> SKGENSKLNPWAVVGFIDAEGSFMVRVRKNSKYKTGWLVVAIFSVTVDKKDLFLLESLKTFFGGLGSIKKSGNSTFSYRIESSEQLTKIILPFFDKYSLITEKLGDYLLFKKVLELMGTKEHLTQRGLEKIVSLKASINKGLSEELQAAFPQCVPTPRPEINNKNIPDPFWLAGFV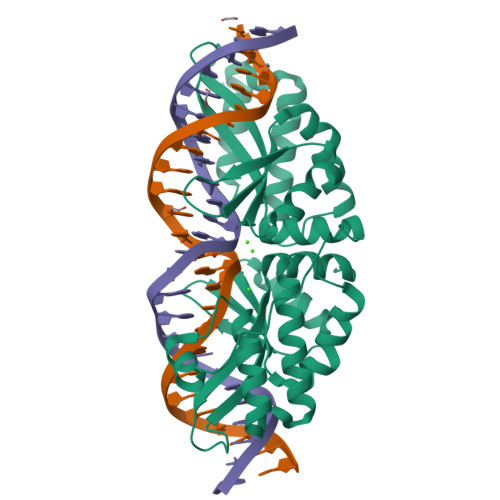SGDGSFKSILKKSESIKVGFQSILVFQITQHARDVKLMESLISYLGCGFIEKDSRGPWLYYTVTNFSDIQGKIIPFFHQYKIIGSKYGDYMDWCKIALIMQNKNHLTPEGLNEIRALKGGMNKGRL> 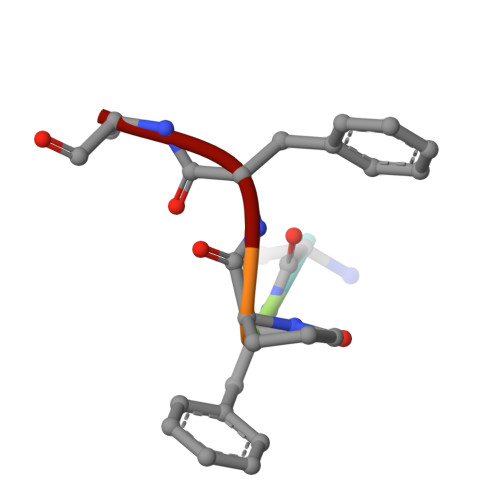DFPFV> MWEQQRPRRCEAPA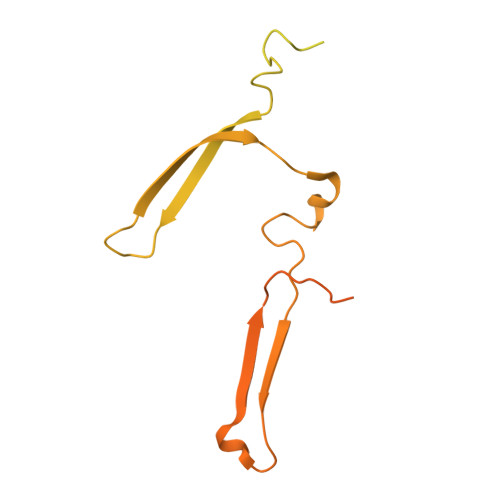APSSRPAERRAAARRSRAQLRMKQDDYEQWKTEFAGGFPGGEAFYKKWIEEGAKGDVPALEEELQPRSPNKKPTIYEEQMISNRGQQKGVDPTWKTLLAGGFPGGEFFFKKWIGEGAQGEVPNLDADLQPGSGSAKKTGKKEDADKSSPGGIMTPGRIMVPSGLGEEEETVDKEAPRPELYNKYFSADRLHKAPEILFEYNKTKYDRVGVRYTEVTSKASERFFPKSRMNRAPVIEISYREGAVSTASVSLSMPEISGPPALPFPVPKGDVTTTMVTDPTTGRLKLEFKVDGAAVSAYSDPRATEAYNKMIRK>[5x]YKDDDDKLHSQANLMRLKSDLFNRSPMYPGPTKDDPLTVTLGFTLQDIVKADSSTNEVDLVYWEQQRWKLNSLMWDPNEYGNITDFRTSAADIWTPDITAY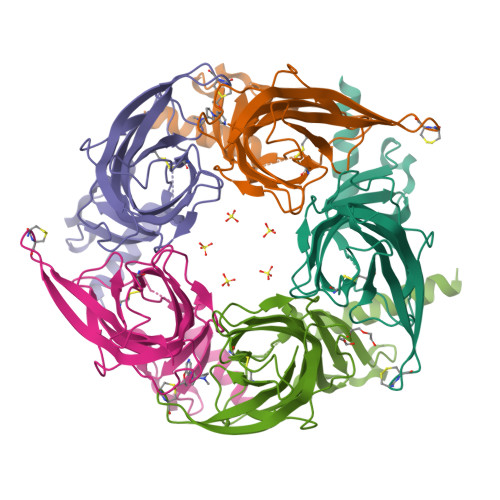SSTRPVQVLSPQIAVVTHDGSVMFIPAQRLSFMCDPTGVDSEEGATCAVKFGSWVYSGFEIDLKTDTDQVDLSSYYASSKYEILSATQYKHDIKYNCCEEIYPDVVLVVKFRERRAGNGFFRNLFDSR> HSTEEGLFSQKSFLVLGFSNENESNIANIIKENAGKIMSLLSRTVADYAVVPLLGCEVEATVGEVVTNTWLVTCIDYQTLFDPKSNPLFTPVPVMTGMTPLEDCVISFSQCAGAE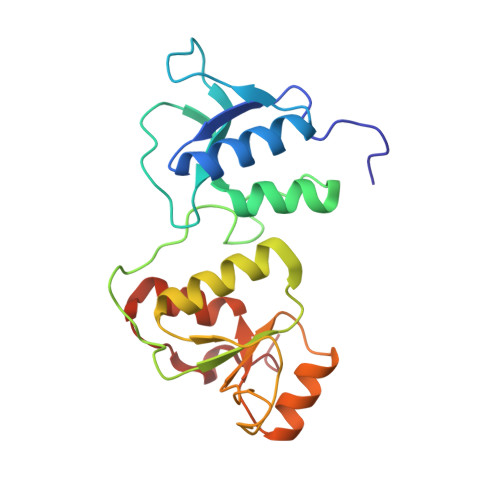KESLTFLANLLGASVQEYFVRKSNAKKGMFASTHLILKERGGSKYEAAKKWNLPAVTIAWLLETARTGKRADESHFLIENS>[4x]MGSHHHHHHGRSAAGTMANLDK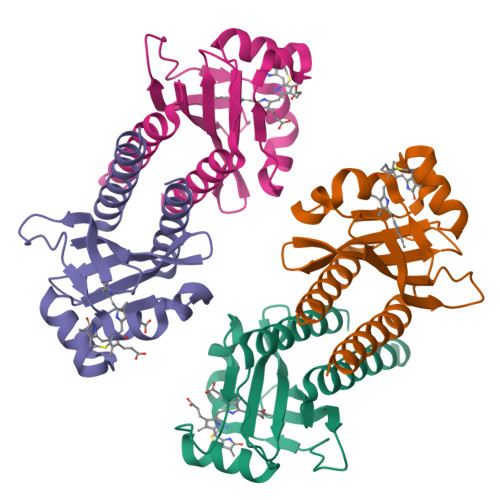MLNTIVTEVRQFLQVDRLCVFKFEEDYSGNIIYEAVDDGWLSILKTHVRDCYFMETRGEEYLHGRYQAIADIHQANLAESYRDFLTQYQVRAIVAVPILKGKKLWGLFSAHQLAAPRSWQAWEIEFLKQQAVVMGIAIQQS>[2x]MTGTVSRRKKIAMIGSGMIGGTMGYLCVLRELADVVLFDVVTGMPEGKALDDSQATSIADTNVSVTSANQYEKIAGSDVVIITAGLTKVPGKSDKEWSRNDLLPFNAKIIREVAQGVKKYCPLAFVIVVTNPLDCMVKCFHEASGLPKNMVCGMANVLDSARFRRFIADQLEISPRD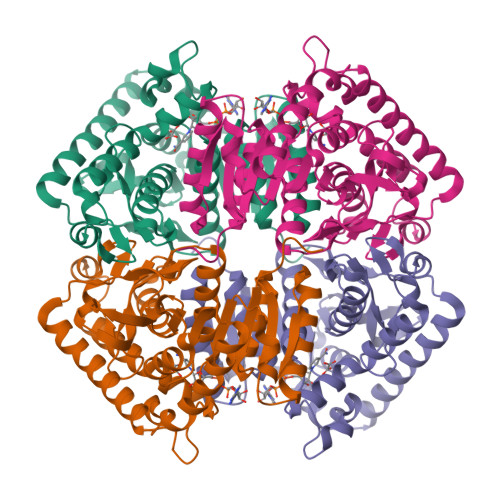IQATVIGTHGDHMLPLARYVTVNGFPLREFIKKGKMTEAKLAEIVERTKKAGGEIVRLLGQGSAYYAPALSAITMAQAFLKDEKRVLPCSVYCQGEYGLHDMFIGLPAVIGGGGIEQVIELELTHEEQECFRKSVDDVVELNKSLAALGPG>[2x]GLVPRGS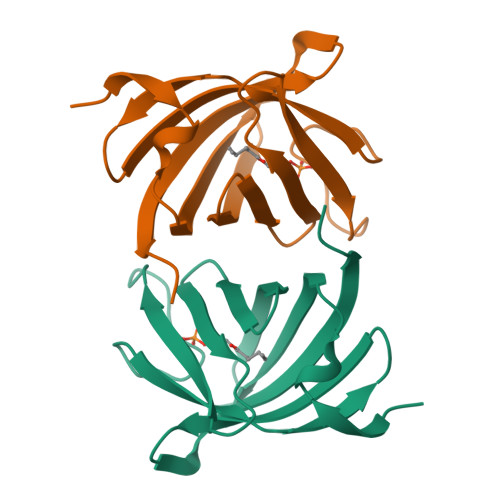MIMKDGIYSIIFISNEDSCGEGILIKNGNMITGGDIASVYQGVLSEDEDIILHVHRYNYEIPSVLNIEQDYQLVIPKKVLSNDNNLTLHCHVRGNEKLFVDVYAKFIEPLV(1'R,2'S)-9-(2-HYDROXY-3'-KETO-CYCLOPENTEN-1-YL)ADENINE | C10 H11 N5 O2 | 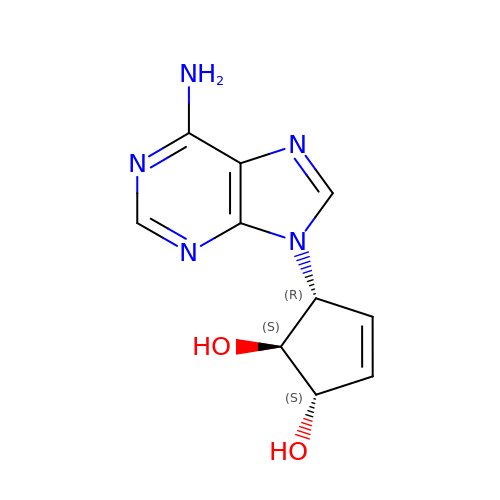RQPALADHFYHEHK-CHKWXVPMSA-N>[6x]MRGSHHHHHHGMSCSKSVIKEEMLIDLHLEGTFNGHYFEIKGKGKGQPNEGTNTVTLEVTKGGPLPFGWHILCPQFQYGNKAFVHHPDNIH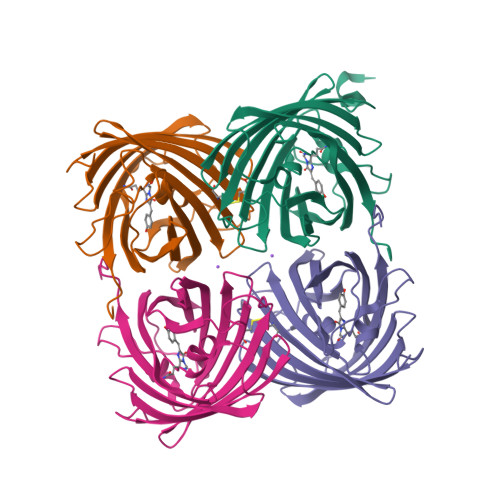DYLKLSFPEGYTWERSMHFEDGGLCCITNDISLTGNCFYYDIKFTGLNFPPNGPVVQKKTTGWEPSTERLYPRDGVLIGDIHHALTVEGGGHYACDIKTVYRAKKAALKMPGYHYVDTKLVIWNNDKEFMKVEEHEIAVARHHPFYEPKKDK>MQPAQDTGNVTNEITIKDIVIYPDAYSIKKRGEDIELTHREFELFHYLSKHMGQVMTREHLLQTVWGYDYFGDVRTVDVTIRRLREKIEDDPSHPEYIVTRRGVGY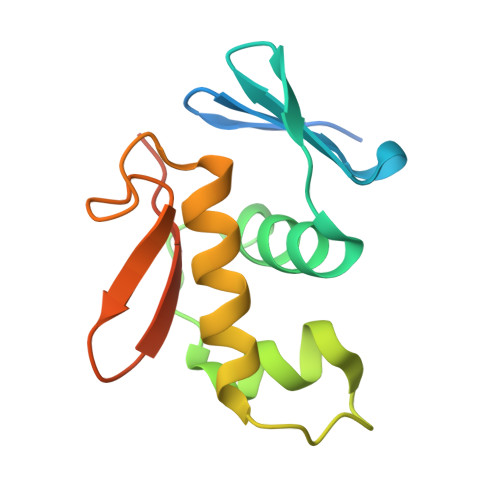FLQQHELEHHHHHH[2x]> DDVTVVYQNGLPVISVRLPSRRERCQFTLKPISDSVGVFLRQLQEEDRGIDRVAIYSPDGVRVAASTGIDLLLLDDFKLVINDLTYHVRPPKRDLLSHENAATLNDVKTLVQQLYTTLCIEQHQLNKERELIERLEDLKEQLAPLEKVRIEISRKAEKRTTLVLWGGLAYMATQFGILARLTWWEYSWDIMEPVTYFIT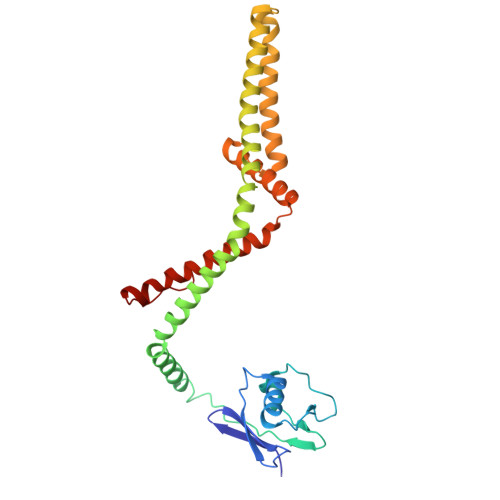YGSAMAMYAYFVMTRQEYVYPEARDRQYLLFFHKGAKKSRFDLEKYNQLKDAIAQAEMDLKRLRDPLQVHLPLRQIG>RSMAEEVSTLMKATVLMRQPGRVQEIVGALRKGGGDRLQVISDFDMTLSRFAYNGKRCPSSYNILDNSKIISEECRKELTALLHHYYPIEIDPHRTVKEKLPHMVEWWTKAHNLLC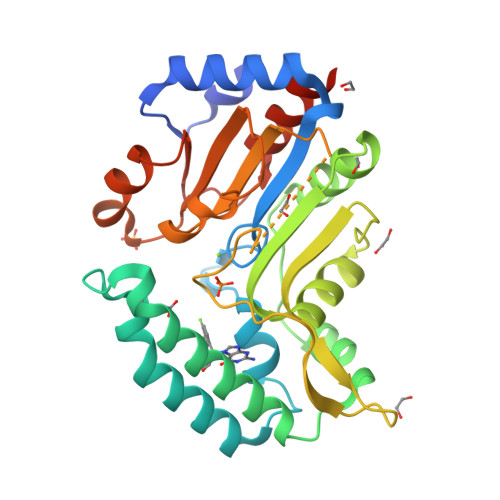QQKIQKFQIAQVVRESNAMLREGYKTFFNTLYHNNIPLFIFSAGIGDILEEIIRQMKVFHPNIHIVSNYMDFNEDGFLQGFKGQLIHTYNKNSSACENSGYFQQLEGKTNVILLGDSIGDLTMADGVPGVQNILKIGFLNDKVEERRERYMDSYDIVLEKDETLDVVNGLLQHILCQGVQLEMQGP[4x]> ADIPANVDGARIIAADKEPGNWMSTGRTYDEQRYSPLKQISDQNVGQLGLAWSYKLDLDRGVEATPIVVDGVMYTTGPFSVVYALDARDGRLIWKYDPQSDRHRAGEACCDAVNRGVAVWKGKVYVGVLDGRLEAIDAKTGQRAWSVDTRADHKRSYTITGAPRVVNGKVVIGNGGAEFGVRGYVTAYDAETGKEAWRFYTVPGDPKLPPEGKGMEIAAKTWFGDAYVEQGGGGTAWDSFAYDPELNLLYIGVGNGSLWDPKWRSQAKGDNLFLSSIVAVNADTGEYVWHYQTTPGDAWDYTATQHMILAELPIDGKPRKVLMQAPKNGFFYVIDR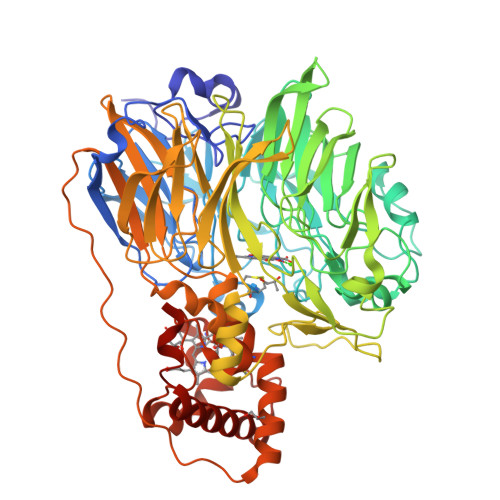ATGELLSAKGIVPQSWTKGMDMKTGRPILDEENAAYWKNGKRNLVTPAFWGAHDWQPMSYNPDTGLVYIPAHIMSAYYEHIPEAPKRNPFKSMYQLGLRTGMMPEGAEGLLEMAKSWSGKLIAWDPVKQQAAWEVPYVTIFNGGTLSTAGNLVFEGSADGRVIAYAADTGEKLWEQPAASGVMAAPVTYSVDGEQYVTFMAGWGGAFSTFAGALSLRAGVQPYAQVLTYKLGGTAKLQEPAPRPDTPKPPALSNDTASIEAGAKLYDGYCSQCHGIHAVSGGVLPDLRKLTPEKHQMFLGILFGGRVPDGMPSFADAFTPEQVDQIHQYLIKRAHDLHQEGDTWKQFSAKSSH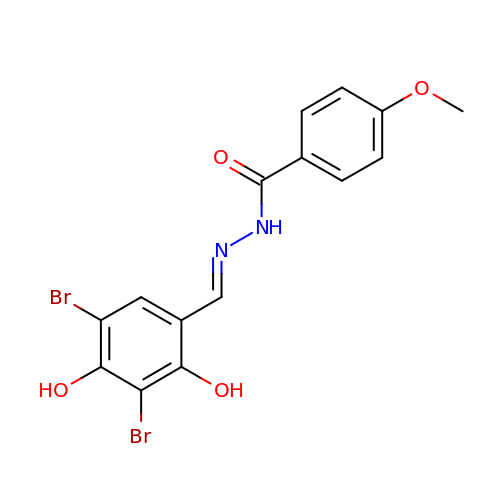N'-[(1E)-(3,5-dibromo-2,4-dihydroxyphenyl)methylidene]-4-methoxybenzohydrazide | C15 H12 Br2 N2 O4 | BMGXNERTVNWBJG-CNHKJKLMSA-N> METLVRPKPELLKLLKSVGAQKDTYTMKEVLFYLGQYIMTKRLYDEKQQHIVYCSNDLLGDLFGVPSFSVKEHRKIYTMI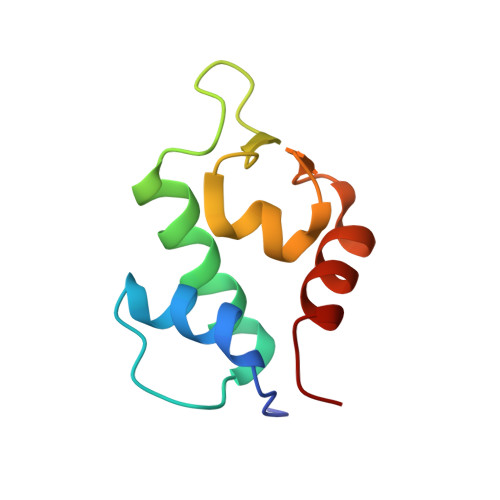YRNLVV The mbd cluster encodes the anaerobic degradation of 3-methylbenzoate in the β-proteobacterium Azoarcus sp. CIB. The three-dimensional structure of MbdR has been solved revealing a conformation similar to that of other TetR family transcriptional regulators. The members of the TetR family are mostly repressors, and MbdR behaves also as a transcriptional repressor of the mbd genes responsible for the anaerobic catabolism of 3-methylbenzoate. In vivo and in vitro experiments revealed that 3-methylbenzoyl-CoA, the first intermediate of the mbd catabolic pathway, is the cognate inducer molecule that interacts with the MbdR repressor allowing transcription from the PO and PB1 promoters.

The crystal structure of MbdR was determined using multiple wavelength anomalous diffraction data, and it was refined to 1.76 Å resolution. The crystal structure reveals that the crystallographic asymmetric unit contains a monomer of the protein. The N-terminal 14 amino acids, residues Thr-46 and Lys-47, and the C-terminal 10 residues in the structure are disordered. Helices α1 to α3 (Ala-13 to Phe-54) make up the N-terminal DNA binding domain and contain the helix-turn-helix motif. The larger C-terminal ligand binding domain of MbdR consists of helices α4 to α9 (Lys-57 to Val-204). A 2-fold crystallographic symmetry operator (arises in space group I222) sits parallel to α4 and generates a dimeric arrangement. The dimer interface is formed mainly by helices α8 and α9 with small contributions from helices α6 and α7. In total, the dimer buries 1759 Å2/monomer of surface area with mostly hydrophobic residues. An electrostatic surface representation of the MbdR dimer structure shows a positively charged patch at the N-terminal domain of both monomers, which might contact the phosphate backbone of the target operator region as in the cases of other TetR family proteins. Binding of 3-methylbenzoyl-CoA would require the movements of helices α5, α6, α8, and α9 in MbdR, similar to that described as the “induced fit” mechanism of QacR bound to its ligand.

> MRKLNKKEEQRKASTENILGCALDLFVKNGYRATTIDMIAARAGLTKGAIYFYFKTKDAIMLMLLEEAEKYIVDPIDEYMANAGPLADAKLVKFINMQALLGVTKPQHVLLLILVSIDFSGTGDDIEKRAKAIYRRMYGHVEQLIAQGQTEGVFRSDSGSDELASIVMAAHDGVLIEWYRRPNELTGKTLTKALRSVLLNGLIVDRGSCKNPTF> MKMANHPRPGDIIQESLDELNVSLREFARAMEIAPSTA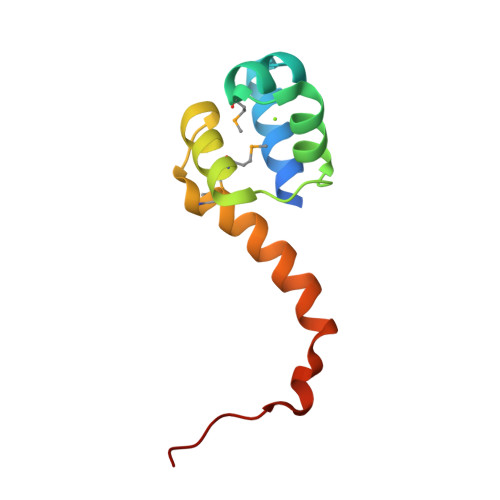SRLLTGKAALTPEMAIKLSVVIGSSPQMWLNLQNAWSLAEAEKTVDVSRLRRLVTQ>[2x]MSGKLTVITGPMYSGKTTELLSFVEIYKLGKKKVAVFKPKIDSRYHSTMIVSHSGNGVEAHVIERPEEMRKYIEEDTRGVFIDEVQFFNPSL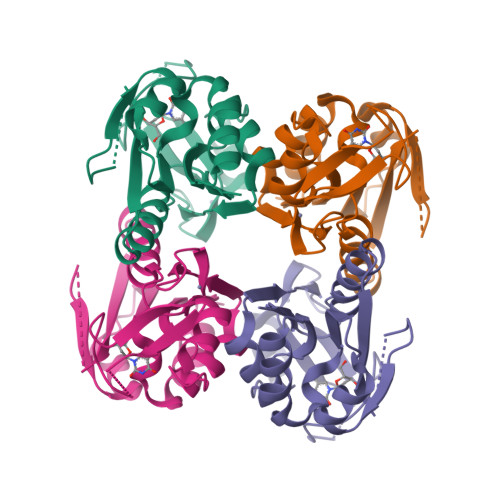FEVVKDLLDRGIDVFCAGLDLTHKQNPFETTALLLSLADTVIKKKAVCHRCGEYNATLTLKVAGGEEEIDVGGQEKYIAVCRDCYNTLKKRV>APAAVDWRARGAVTAVKDQGQCGSCWAFSAIGNVECQWFLAGHPLTNLSEQMLVSCDKTDSGCSGGLMNNAFEWIVQENNGAVYTEDSYPYASGEGISPPCTTSGHTVGATITGHVELPQDEAQIAAWLAVNGPVAVAVDASSWMTYTGGVMTSCVSEQL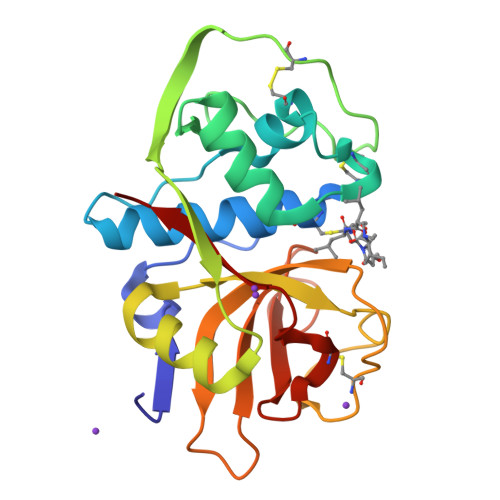DHGVLLVGYNDSAAVPYWIIKNSWTTQWGEEGYIRIAKGSNQCLVKEEASSAVVG[6x]>[2x]GPHMLEMPDEMRAEVLARNEISNLIMDAAEAAQHALPLEVENYHALYPLEPPAQPLHAKLTFPATTYRATHNTTGYKYCLRRIHGFRLQSTKCMTLVEMWKKLQHTNVVQLREVFTTKAFGDNSLVLVYDYHPGSQTLLAKYFTPAPETNGYTDPFQGEARPFSHKSNMQRTSNGPLLPEATIWSIIMQLTAGLKAIHHAGLACKVLDPTKIIVTGKRVRFSSCCISDITQFDPNASNPLALVNMHQ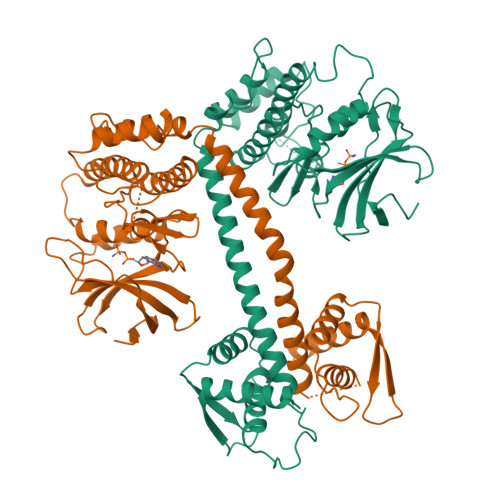QDDLTALGRLVLALACRCLQSVQRDNVQSSIDMVTRNYSTDLRNFIVYLFTTNNRRSVTDLMPMIGARFYTQLDALQSKIDMQEDELAKEMENGRLYRILVKLNSINERPDFNLDCTWSETGDRYMLKLFRDYLFHSVTEDGRPWLDHAHIVQCLNKLDAGSIERVQLMSRDEQSVLIVSYAELKNCLENAFSELMSSAAN> MSITTPEE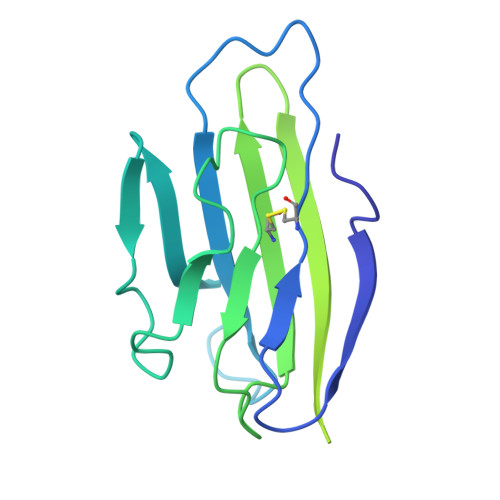MIEKAKGETAYLPCKFTLSPEDQGPLDIEWLISPADNQKVDQVIILYSGDKIYDDYYPDLKGRVHFTSNDLKSGDASINVTNLQLSDIGTYQCKVKKAPGVANKKIHLVVLVKPSGARCYVDGSEEIGSDFKIKCEPKEGSLPLQYEWQKLSDSQKMPTSWLAEMTSSVISVKNASSEYSGTYSCTVRNRVGSDQCLLRLNVVPPSNKALEHHHHHH>SNAMIVGLGTDIAEIERVEKALARSGENFARRILTDSELEQFHASKQQGRFLAKRFAAKEAASKALGTGIAQGVTFHDFTISHDKLGKPLLILSGQAAELASQLQVENIHLSISDERHYAMATVILERR[24x]

The active form of ACP is produced by a post-translational modification of a conserved serine residue of apo-ACP by a 4′-phosphopantetheine (P-pant) group transferred from CoA bound to a holo-(acyl-carrier-protein) synthase (AcpS). AcpS belongs to the phosphopantetheine transferase (PPT) family of proteins, binds CoA and its derivatives and requires magnesium for activity. The AcpS trimer binds three CoA molecules and three ACP molecules. The AcpS monomer has an elongated elliptical shape and possesses an α/β fold.

24 polypeptide chains of AcpSVC are arranged in eight trimers in the P21 asymmetric unit. Three molecules of CoA were modeled per trimer. The pantothenate parts of all CoAs have two kinks of ∼100–110° that might be forced by intramolecular and intermolecular protein–ligand contacts. The high thermal factors and observed conformational diversity of the P-pant moiety can be explained by the mechanism of the reaction, in which accessibility of the group is essential. Whether the purification tag was present or absent, crystals of apo-AcpSBA and apo-AcpSVC only diffracted to low resolution.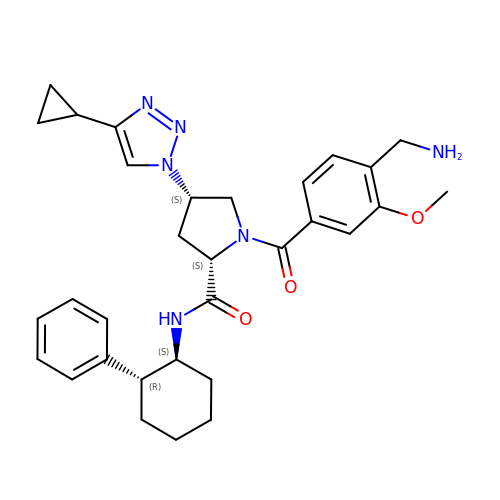(2~{S},4~{S})-1-[4-(aminomethyl)-3-methoxy-phenyl]carbonyl-4-(4-cyclopropyl-1,2,3-triazol-1-yl)-~{N}-[(1~{S},2~{R})-2-phenylcyclohexyl]pyrrolidine-2-carboxamide | C31 H38 N6 O3 | AYVQDWAWTUYBGU-RVUATISTSA-N5-(2-chlorophenyl)furan-2-carbohydrazide | C11 H9 Cl N2 O2 | 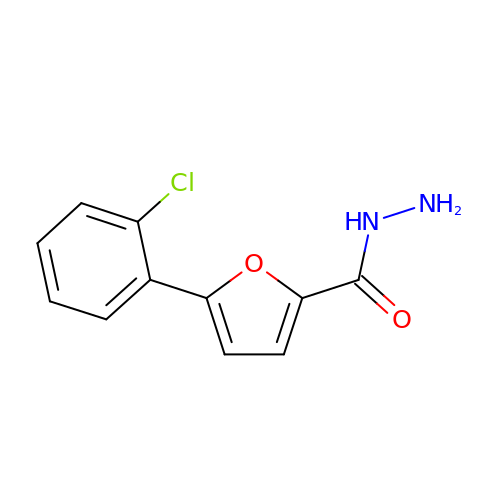XQMRHWSGTVEDFG-UHFFFAOYSA-N[(1S)-1-{[(2,6-DIMETHOXYPHENYL)CARBONYL]AMINO}ETHYL]BORONIC 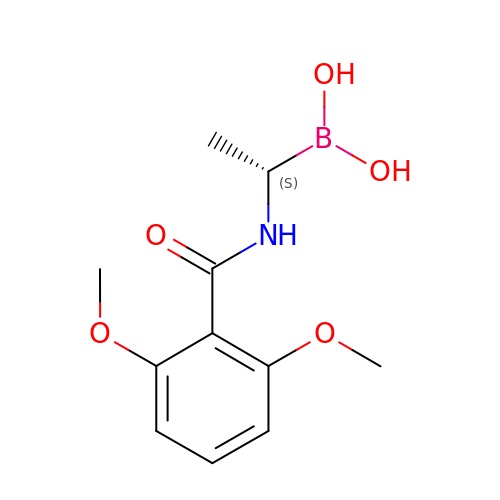ACID | C11 H16 B N O5 | DXKXQRZEPYKFAT-SSDOTTSWSA-N>[4x]MLSRKGIIPEEYVLTRLAEDPAKPRYRARQRRARFVSKKGNCNVAHKNIREQGRFLQDVFTTLVDLKWPHTLLIFTMSFLCSWLLFAMAWWLIAFAHGDLAPSEGTAEPCVTSIHSFSSAFLFSIEVQVTIGFGGRMVTEECPLAILILIVQNIVGLMINAIMLGSIFMKTAQAHRRAETLIFSKHAVIALRHGRLCFMLRVGDLRKSMIISATIHMQVVRKTTSPEGEVVPLHQVDIPMENGVGGNSIFLVAPLIIYHVIDANSPLYDLAPSDLHHHQDLEIIVILEGVVETTGITTQARTSYLA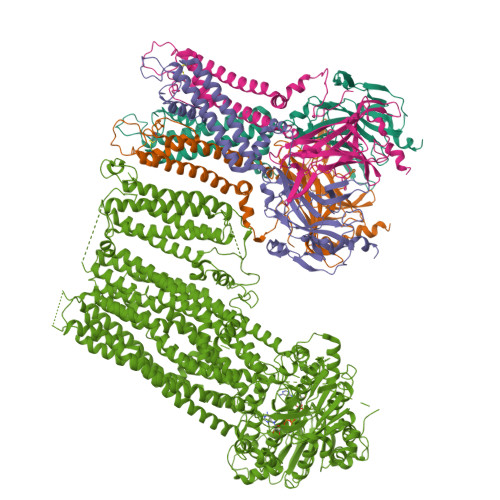DEILWGQRFVPIVAEEDGRYSVDYSKFDNTVKVPTPLCTARQLDEDHSLLEALTLASARGPLRKRSVPMAKAKPKFSISPDSLS;> MGPLAFCGSENHSAAYRVDQGVLNNGCFVDALNVVPHVFLLFITFPILFIGWGSQSSKVHIHHSTWLHFPGHNLRWILTFMLLFVLVCEIAEGILSDGVTESHHLHLYMPAGMAFMAAVTSVVYYHNIETSNFPKLLIALLVYWTLAFITKTIKFVKFLDHAIGFSQLRFCLTGLLVILYGMLLLVEVNVIRVRRYIFFKTPREVKPPEDLQDLGVRFLQPFVNLLSKGTYWWMNAFIKTAHKKPIDLRAIGKLPIAMRALTNYQRLCEAFDAQVRKDIQGTQGARAIWQALSHAFGRRLVLSSTFRILADLLGFAGPLCIFGIVDHLGKENDVFQPKTQFLGVYFVSSQEFLANAYVLAVLLFLALLLQRTFLQASYYVAIETGINLRGAIQTKIYNKIMHLSTSNLSMGEMTAGQICNLVAIDTNQLMWFFFLCPNLWAMPVQIIVGVILLYYILGVSALIGAAVIILLAPVQYFVATKLSQAQRSTLEYSNERLKQTNEMLRGIKLLKLYAWENIFRTRVETTRRKEMTSLRAFAIYTSISIFMNTAIPIAAVLITFVGHVSFFKEADFSPSVAFASLSLFHILVTPLFLLSSVVRSTVKALVSVQKLSEFLSSAEIREEQCAPHEPTPQGPASKYQAVPLRVVNRKRPAREDCRGLTGPLQSLVPSADGDADNCCVQIMGGYFTWTPDGIPTLSNITIRIPRGQLTMIVGQVGCGKSSLLLAALGEMQKVSGAVFWSSLPDSEIGEDPSPERETATDLDIRKRGPVAYASQKPWLLNATVEENIIFESPFNKQRYKMVIEACSLQPDIDILPHGDQTQIGERGINLSGGQRQRISVARALYQHANVVFLDDPFSALDIHLSDHLMQAGILELLRDDKRTVVLVTHKLQYLPHADWIIAMKDGTIQREGTLKDFQRSECQLFEHWKTLMNRQDQELEKETVTERKATEPPQGLSRAMSSRDGLLQDEEEEEEEAAESEEDDNLSSMLHQRAEIPWRACAKYLSSAGILLLSLLVFSQLLKHMVLVAIDYWLAKWTDSALTLTPAARNCSLSQECTLDQTVYAMVFTVLCSLGIVLCLVTSVTVEWTGLKVAKRLHRSLLNRIILAPMRFFETTPLGSILNRFSSDCNTIDQHIPSTLECLSRSTLLCVSALAVISYVTPVFLVALLPLAIVCYFIQKYFRVASRDLQQLDDTTQLPLLSHFAETVEGLTTIRAFRYEARFQQKLLEYTDSNNIASLFLTAANRWLEVRMEYIGACVVLIAAVTSISNSLHRELSAGLVGLGLTYALMVSNYLNWMVRNLADMELQLGAVKRIHGLLKTEAESYEGLLAPSLIPKNWPDQGKIQIQNLSVRYDSSLKPVLKHVNALIAPGQKIGICGRTGSGKSSFSLAFFRMVDTFEGHIIIDGIDIAKLPLHTLRSRLSIILQDPVLFSGTIRFNLDPERKCSDSTLWEALEIAQLKLVVKALPGGLDAIITEGGENFSQGQRQLFCLARAFVRKTSIFIMDEATASIDMATENILQKVVMTAFADRTVVTIAHRVHTILSADLVIVLKRGAILEFDKPEKLLSRKDSVFASFVRADK>ENMAVQSPKKHVFDAVIKAYKDNSDEESYATVYIKDPKLTIENGKR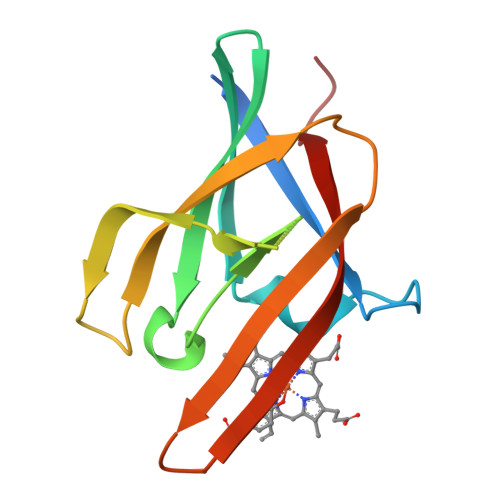IITATLKDSDFFDYLKVEDSKEPGVFHDVKVLSEDKRKHGTKVIQFEVGELGKRYNMQMHILIPTLGYDKEFKIQFEVNMRTFV[2x]> LPTSNPAQELEARQLGRTTRDDLINGNSASCRDVIFIYARGATETGNLGTLGPSIASNLESAFGKDGVWIQGVGGAYRATLGDNALPRGTSSAAIREMLG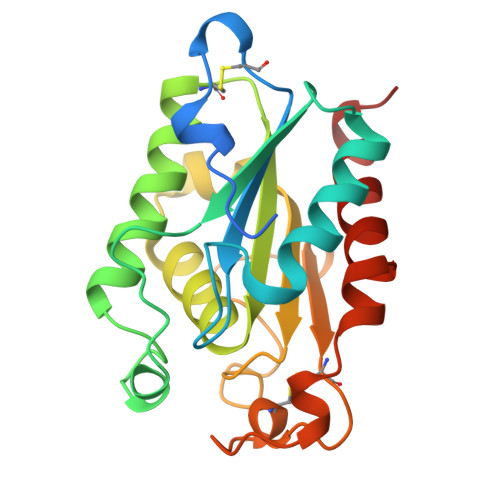LFQQANTKCPDATLIAGGYSQGAALAAASIEDLDSAIRDKIAGTVLFGYTKNLQNRGRIPNYPADRTKVFCNTGDLVCTGSLIVAAPHLAYGPDARGPAPEFLIEKVRAVRGSA> ACGCAGCCTGTACG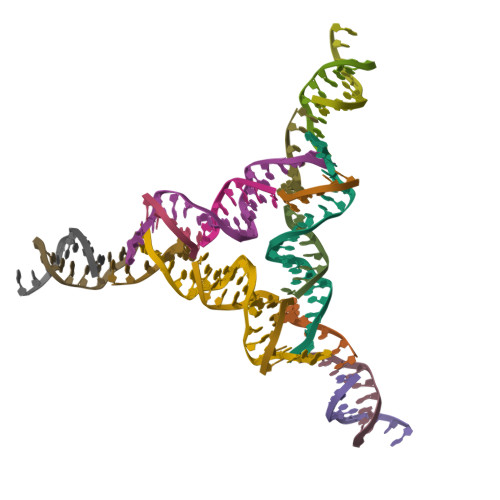GACATCA;> CCGTACA;> GGCTGC;> TCTGATGT;> GATGCGAGT;> GTACTCGCA> SVGGIISQSFFNGLAGGAASSCEGKGFYTYNAFIAAANAYSGFGTTGSNDVKKRELA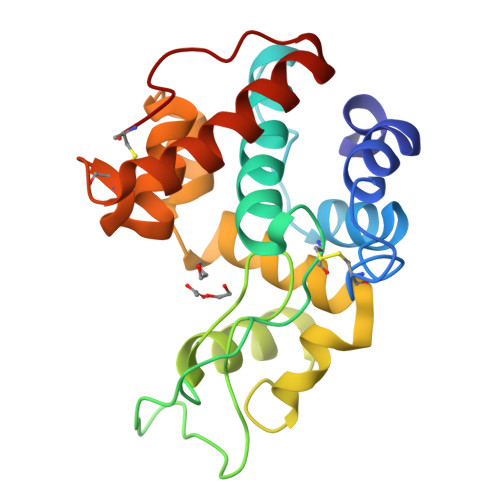AFFANVMHETGGLCYINEKNPPINYCQSSSTWPCTSGKSYHGRGPLQLSWNYNYGAAGKSIGFDGLNNPEKVGQDSTISFKTAVWFWMKNSNCHSAITSGQGFGGTIKAINSMECNGGNSGEVSSRVNYYKKICSQLGVDPGANVSC>MFNQFNPLVYTHGGKLERKSKKDKTASKVFEEFGVMEAYNCWKEASLCIQQRDKDSVLKLVAALNTYKDAVEPIFDSRLNSAQEVLQPSILEEFFEYLFSRIDSIVGVNIPIRHPAKGYLSLSFNPHNIETLIQSPEYTVRAKDHDFIIGGSAKLTIQGHGGEGETTNIVVPAVAIECKRYLERNMLDECAGTAERLKRATPYCLYFVVAEYLKLDDGAPELTEIDEIYILRHQRNSERNKPGFKPNPIDGELIWDLYQEVMNHLGKIWWDPNSALQRGKVFNRP[2x]

BbvCI, a Type IIT restriction endonuclease, recognizes and cleaves the seven base pair sequence 5′-CCTCAGC-3′, generating 3-base, 5′-overhangs. BbvCI is composed of two protein subunits, each containing one catalytic site. Either site can be inactivated by mutation resulting in enzyme variants that nick DNA in a strand-specific manner. Earlier mutagenesis of these residues confirmed their catalytic nature and demonstrated that the site in the R1 subunit cleaves the bottom strand of the target site, while the site in the R2 subunit cleaves the top strand.

Purified samples of wild-type BbvCI, containing a 1:1 ratio of R1 and R2 subunits yielded crystals under acidic conditions (pH 4.5) in the presence of an excess of duplex DNA oligo containing the target site, and 2 mM calcium chloride. However, after derivatization with heavy atom compounds ‘I3C’ or tantalum bromide, the space group was converted to C2221, with only two subunits (one dimer) in the asymmetric unit. We initially calculated MIR phases, built an initial structure, and conducted refinements using datasets corresponding to the latter (heavy-atom) space group, and then subsequently determined the final, higher resolution structure of the native (non-derivatized) protein in the original C222 space group via molecular replacement and phase extension. The resulting electron density maps clearly corresponded to two full-length protein chains, but no density corresponding to DNA was present. In contrast, modeling the electron density as a homodimer comprising two copies of the R2 subunit resulted in satisfactory values for Rwork and Rfree (0.189/0.249, respectively), excellent correlation of the model to experimental electron density, and significantly improved geometric quality. An intervening four-stranded, anti-parallel beta-sheet (residues 116–175) protrudes from this core. This interacts in a domain-swapped manner with its symmetry-mate in the opposing subunit, to form a dimer interface corresponding to an elongated beta-sheet. However, the two sites in the protein dimer are located ∼45 Å apart from one another–too far away from each other to catalyze double-strand cleavage reactions producing a 3-base overhang.>[2x]MHHHHHHGRIGIPRERLTNETRVAAT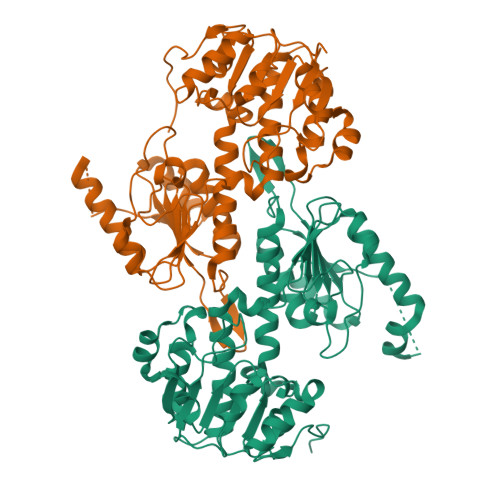PKTVEQLLKLGFTVAVESGAGQLASFDDKAFVQAGAEIVEGNSVWQSEIILKVNAPLDDEIALLNPGTTLVSFIWPAQNPELMQKLAERNVTVMAMDSVPRISRAQSLDALSSMANIAGYRAIVEAAHEFGRFFTGQITAAGKVPPAKVMVIGAGVAGLAAIGAANSLGAIVRAFDTRPEVKEQVQSMGAEFLELDFKEEAGSGDGYAKVMSDAFIKAEMELFAAQAKEVDIIVTTALIPGKPAPKLITREMVDSMKAGSVIVDLAAQNGGNCEYTVPGEIFTTENGVKVIGYTDLPGRLPTQSSQLYGTNLVNLLKLLCKEKDGNITVDFDDVVIRGVTVIRAGEITWPAPPIQVSAQPQAAQKAAPEVKTEEK>KPRKARTAFSDHQLNQLERSFERQKYLSVQDRMDLAAALNLTDTQVK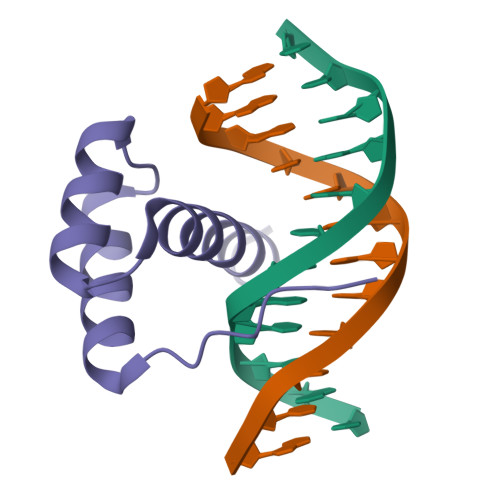TWYQNRRTKWKRQTA[4x]>GAMGSMWKRSEQMKIKSGKCNMAAAMETEQLGVEIFETADCEENIESQDRPKLEPFYVERYSWSQLKKLLADTRKYHGYMMAKAPHDFMFVKRNDPDGPHSDRIYYLAMSGENRENTLFYSEIPKTINRAAVLMLSWKPLLDLFQATLDYGMYSREEELLRERKRIGTVGIASYDYHQGSGTFLFQAGSGIYHVKDGGPQGFTQQPLRPNLVETSCPNIRMDPKLCPADPDWIAFIHSNDIWISNIVTREERRLTYVHNELANMEEDARSAGVATFVLQEEFDRYSGYWWCPKAETTPSGGKILRILYEENDESEVEIIHVTSPMLETRRADSFRYPKTGTANPKVTFKMSEIMIDAEGRIIDVIDKELIQPFEILFEGVEYIARAGWTPEGKYAWSILLDRSQTRLQIVLISPELFIPVEDDVMERQRLIESVPDSVTPLIIYEETTDIWINIHDIFHVFPQSHEEEIEFIFASECKTGFRHLYKITSILKESKYKRSSGGLPAPSDFKCPIKEEIAITSGEWEVLGRHGSNIQVDEVRRLVYFEGTKDSPLEHHLYVVSYVNPGEVTRLTDRGYSHSCCISQHCDFFISKYSNQKNPHCVSLYKLSSPEDDPTCKTKEFWATILDSAGPLPDYTPPEIFSFESTTGFTLYGMLYKPHDLQPGKKYPTVLFIYGGPQVQLVNNRFKGVKYFRLNTLASLGYVVVVIDNRGSCHRGLKFEGAFKYKMGQIEIDDQVEGLQYLASRYDFIDLDRVGIHGWSYGGYLSLMALMQRSDIFRVAIAGAPVTLWIFYDTGYTERYMGHPDQNEQGYYLGSVAMQAEKFPSEPNRLLLLHGFLDENVHFAHTSILLSFLVRAGKPYDLQIYPQERHSIRVPESGEHYELHLLHYLQENLGSRIAALKVI[3x];>SLRFLFEGQRIADNH[3x]

Here we present the development and application of the Aerosol-Generator (AeGe), a new gentle soaking device that complements the humidity control and uses ultrasonic vibration to generate aerosols of ligands to soak reservoir-free protein crystals. The AeGe technique uses reservoir-free crystals under a temperature/humidity-controlled gas stream. In other words, ligands are directly soaked into protein crystals without being diluted in the crystallization drop. Two protein model systems confirm the advantages of using the AeGe method in challenging complex formation scenarios.

We tested the AeGe on dipeptidyl peptidase (DPP8) crystals using two ligands which evaded complex formation by regular soaking methods. Both 1G244 and the E67-interacting loop (EIL) peptide (SLRFLFEGQRIADNH) are inhibitors of DPP8 and DPP9. 1G244 is a model for a water-insoluble mol­ecule and the EIL peptide is a model for a low-affinity binder: neither forms complexes with DPP8 using classical soaking. Similarly, to soak 0.5 mM EIL peptide in a solution of 50 mM TMAO, an r.h. gradient was started at 97.3% with 0.1% steps/45 s down to 80% (2 h 10 min in total) with a gas temperature of 19°C. In contrast to the method employed to soak 1G244 (DMSO soluble), spraying the EIL peptide (water soluble) implies reaching an equilibrium at the end humidity, not crossing the lower optical shrinkage threshold, and thus the dehumidification stops automatically. Given that 4.5 M TMAO is approximately in equilibrium with 80% r.h., the equivalent accumulation of the EIL peptide in this experimental setup was theoretically 90-fold, resulting in 45 mM peptide as the final concentration in the crystal. Similarly, we determined the crystallographic structure of the AeGe-soaked DPP8–SLRFLFEGQRIADNH crystals at 3.0 Å. Strong positive electron density is observed in the active site assigned to the EIL peptide, albeit not complete. Interestingly, the binding mode of the EIL peptide closely resembles that of SLRLFLYEG, first in the anchoring of its N-terminus to two glutamic acids, and second by the induced-fit formation of an S2′ hydro­phobic sub-site to allocate the F4 residue. Moreover, both ligands induced the ordering of the R segment, a common feature of peptide-like binders. However, the reason why the EIL peptide has lower binding affinity compared with SLRFLYEG remains elusive. In fact, the only sequence difference (F to Y) does not provide further clues, since both residues are exposed to solvent without forming strong contacts.>[2x]QYKDNIRHGVCWIYYPDGGSLVGEVNEDGEMTGEKIAYVYPDERTALYGKFIDGEMIEGKLATLMSTEEGRPHFELMPGNSVYHFDKSTSSCIST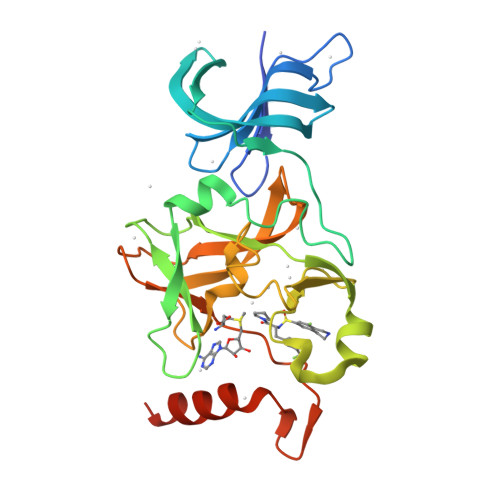NALLPDPYESERVYVAESLISSAGEGLFSKVAVGPNTVMSFYNGVRITHQEVDSRDWALNGNTLSLDEETVIDVPEPYNHVSKYCASLGHKANHSFTPNCIYDMFVHPRFGPIKCIRTLRAVEADEELTVAYGYDHSPPGKSGPEAPEWYQVELKAFQATQQKHHHHHH> AKCVSYGVSQIKAPALHSQGYTGSNVKVAVIDSGIDSSHPDLNVAGGASFVPSETNPFQDNNSHGTHVAGTVLAVAPSASLYAVKVLGADGSGQYSWIINGIEWAIANNMDVINMSLGGPSGSAALKAAVDKAVASGVVVVAAAGNSGTSGSSSTVSYPAKYPSVIAVGAVDSSNQRAPFSSVGPELDVMAPGVSICSTLPGNKYGALSGTCPASAHVAGAAALILSKHPNWTNTQVRSSLENTATKLGDSFYYGKGLINVEAAAQHHHHH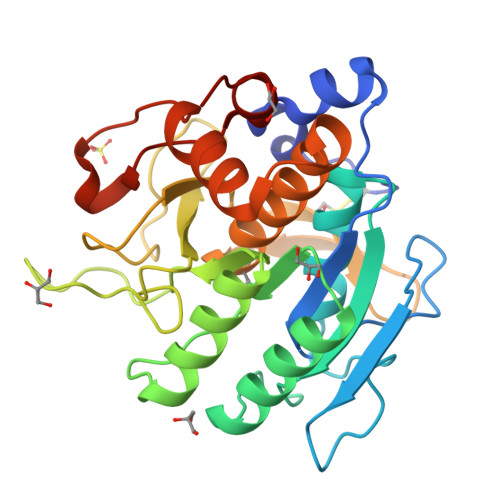H> MIVLENHTDISGKTSERVLHSAWLNSHYQTGLKNLLDTAVLEGTDEESARSLASRWQKIDEIPFDFERRRMSVVVAENTEHHQLVCKGALQEILNVCSQVRHNGE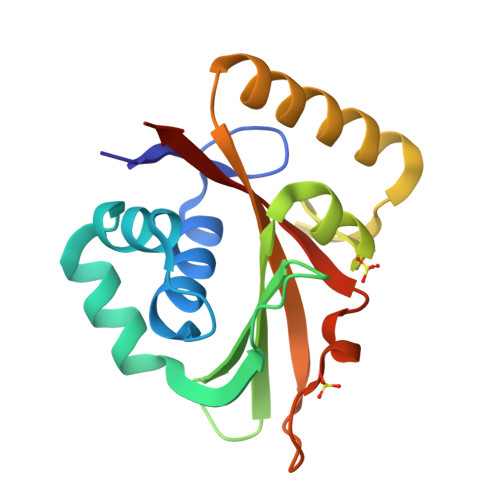IVPLDDIMLRKIKRVTDTLNRQGLRVVAVATKYLPAREGDYQRADESDLILEGYIAFLDHHHHHH>MAHHHHHHSAALEVLF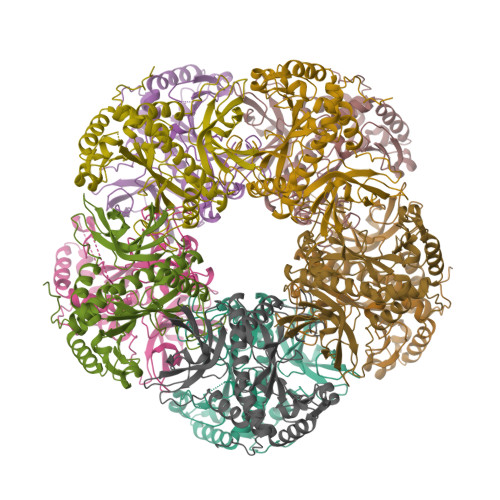QGPGEKVQAMYIWIDGTGEGLRCKTRTLDSEPKCVEELPEWNFDGSSTLQSEGSNSDMYLVPAAMFRDPFRKDPNKLVLCEVFKYNRRPAETNLRHTCKRIMDMVSNQHPWFGMEQEYTLMGTDGHPFGWPSNGFPGPQGPYYCGVGADRAYGRDIVEAHYRACLYAGVKIAGTNAEVMPAQWEFQIGPCEGISMGDHLWVARFILHRVCEDFGVIATFDPKPIPGNWNGAGCHTNFSTKAMREENGLKYIEEAIEKLSKRHQYHIRAYDPKGGLDNARRLTGFHETSNINDFSAGVANRSASIRIPRTVGQEKKGYFEDRRPSANCDPFSVTEALIRTCLLNETGDEPFQYKN[10x]> SIPWNLERITPPRYRADEYQPPDGGSLVEVYLLDTSIQSDHREIEGRVMVTDFENVPEEDGTRFHRQASKCDSHGTHLA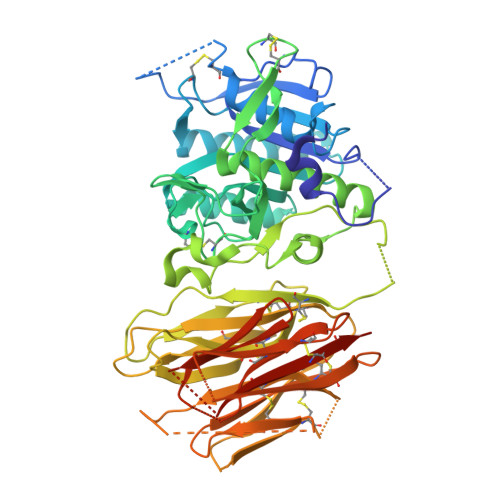GVVSGRDAGVAKGASMRSLRVLNCQGKGTVSGTLIGLEFIRKSQLVQPVGPLVVLLPLAGGYSRVLNAACQRLARAGVVLVTAAGNFRDDACLYSPASAPEVITVGATNAQDQPVTLGTLGTNFGRCVDLFAPGEDIIGASSDCSTCFVSQSGTSQAAAHVAGIAAMMLSAEPELTLAELRQRLIHFSAKDVINEAWFPEDQRVLTPNLVAALPPSTHGAGWQLFCRTVWSAHSGPTRMATAIARCAPDEELLSCSSFSRSGKRRGERMEAQGGKLVCRAHNAFGGEGVYAIARCCLLPQANCSVHTAPPAEASMGTRVHCHQQGHVLTGCSSHWEVEDLGTHKPPVLRPRGQPNQCVGHREASIHASCCHAPGLECKVKEHGIPAPQEQVTVACEEGWTLTGCSALPGTSHVLGAYAVDNTCVVRSRDVSTTGSTSEEAVTAVAICCRSRHLAQASQELQ> VVGGEDAKPGQFPWQVVLNGKVDAFCGGSIVNEKWIVTAAHCVETGVKITVVAGEHNIEETEHTEQKRNVIRIIPHHNYNAAINKYNHDIALLELDEPLVLNSYVTPICIADKEYTNIFLKFGSGYVSGWGRVFHKGRSALVLQYLRVPLVDRATCLRSTKFTIYNNMFCAGFHEGGRDSCQGDSGGPHVTEVEGTSFLTGIISWGEECAMKGKYGIYTKVSRYVNWIKEKTKL;> MDVTC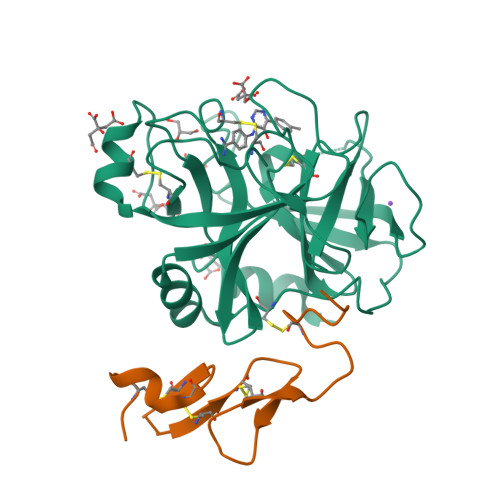NIKNGRCEQFCKNSADNKVVCSCTEGYRLAENQKSCEPAVPFPCGRVSVSQTSKLTR>MPVEKDLKTAYKALYDEKEPLKALHLYDEILKGSPTNLTALIFKAACLEKLYFGFSDWHSDATMENAKELLDKALMTAEGRGDRSKIGLVNFRYFVHFFNIKDYELAQSYFKKAKNLGYVDDTLPLWEDRLETKLNKKNKKQKDSTNKHT[3x];> MVTSNVVLVSGEGERFTVDKKIAERSLLLKNYLNDASGDDDDEDDDEIVMPVPNVRSSVLQKVIEWAEHHRDSNFPDEDDDDSRKSAPVDSWDREFLKVDQEMLYEIILAANYLNIKPLLDAGCKVVAEMI

Sgt1 is an essential conserved cochaperone of the molecular chaperone Hsp90. The N-terminal domain of Sgt1 is predicted to have a helical TPR fold (Tetratrico-Peptide Repeat) and is responsible for the interaction with Skp1. Skp1 has an N-terminal BTB/POZ domain31 that interacts with Cullin1, a structural subunit of the SCF complexes that arranges the substrate and ligase subunits in close proximity, and a C-terminal extension of around 35 residues, that folds around the helices of F-box motifs.

Crystals were obtained that diffracted to 2.8 Å of a complex comprising Sgt1TPR and a truncated construct of Skp1, Skp1BTB∆. The Skp1BTB∆ construct comprises the N-terminal BTB/POZ domain in which an unconserved loop that is predicted to be unstructured (residues 36–64) is replaced by an alanine-serine linker. The asymmetric unit contains 3 copies of Sgt1TPR (chains A, B & C) and a single copy of Skp1BTB∆. The Sgt1 TPR domain comprises 3 TPR motifs, each of two antiparallel helices (A & B), and a solvating helix (κ). Skp1 sits within the upper half of the concave face generated by the Sgt1 TPR motif repeats. Residues from the α2-helix and β3-strand of Skp1BTB∆ form the interface with residues from Sgt1 TPR1A, 2 A, 3 A and the capping helix. In this interface the α2-helix of Skp1BTB∆is amphipathic and forms a bipartite interface with Sgt1 in which half is hydrophobic, and half is electrostatic. A pivotal interaction in this interface is a salt-bridge between Sgt1-Arg93 and Skp1-Asp35, and our structure-guided mutagenesis experiments using full-length proteins show that mutation of Arg93 alone is sufficient to prevent Skp1 binding in vitro and cause loss of viability in vivo. The three copies of Sgt1TPR in the asymmetric unit form two identical dimeric interfaces (between C-A and A-B) with an rmsd of 1.46 Å in an all-atom superposition. The yeast specific insertion between TPR2A and 2B of both protomers contributes the majority of the interactions of this interface.Three salutaridine/menthone reductase like subfamilies of short‐chain dehydrogenases/reductases (SDRs)2 from Mentha piperita were identified, namely (−)‐menthone:(−)‐menthol reductase (MMR), (−)‐menthone:(+)‐neomenthol reductase (MNMR), and isopiperitenone reductase (IPR).1a,1b MMR and MNMR catalyze the ketoreduction of (−)‐menthone 1 a to (1R,2S,5R)‐menthol 2 a and (1S,2S,5R)‐neomenthol 2 b, respectively.1a Additionally, they act on isomenthone 1 b to produce (1R,2R,5R)‐neoisomenthol 2 c and (1R,2S,5S)‐isomenthol 2 d, respectively. Interestingly, the three Mentha SDRs have high protein‐sequence identities (63–68 %), so we performed comparative studies of MMR, MNMR, and IPR, to pinpoint the determinants of ketoreductase vs. ene‐reductase activity within SDRs. A key difference in the sequences between the ketoreductases and IPR was a substitution of the highly conserved catalytic Tyr residue for Glu (238 in IPR). We determined crystal structures of both MNMR and IPR, the latter in combination with NADP+, alkene 3 a, and β‐cyclocitral (non‐substrate).

The MNMR structure was solved by molecular replacement using IPR as the search model (resolution 2.3–2.7 Å), and was found to be structurally similar (rmsd 0.97 Å). Major structural differences were not observed between apoprotein and NADP+‐bound forms. Therefore the bulkier MNMR Tyr 244 likely positions substrates in a different conformation compared to that observed for 3 a in IPR because of the larger side‐chain bulk of tyrosine. This is consistent with the helix of the flap domain (MNMR) being shifted compared to that in IPR, to accommodate binding of 1 a,b. KGaABiotransformations with MMR and MNMR showed only ketoreduction products, with no detectable double bond reduction.1a,1b Reactions with 1 a and 1 b generated the menthol isomers 2 a–d (entries 7, 8, 10, and 11).

> GAMGDEVVVDHAATKRYAVVTGANKGIGFEICKQLASKGITVILASRDEKRGIEARERLIKELGSEFGDYVVSQQLDVADPASVAALVDFIKTKFGSLDILVNNAGLNGTYMEGDASVLNDYVEAEFKTFQSGAAKTEPYHPKATGRLVETVEHAKECIETNYYGSKRVTEALIPLLQQSDSPRIVNVSSTLSSLVFQTNEWAKGVFSSEEGLTEEKLEEVLAEFLKDFIDGKQQEKQWPPHFSAYKVSKAALNAYTRIIAKKYPSFRINAVCPGYTKTDLSYGHGQFTDAEAAEAPVKLALLPQGGPSGCFFFRDEAFCLYLE>GPLGSPEFSKVPKEYRTAVSKAKQYASTVHMSKEELRSQLVSFDKYSQDASDYAVENSGIDYNKQALEKAKQYQDTLSMSPDAIRDQLVSFDKFTQEEADYAVANLK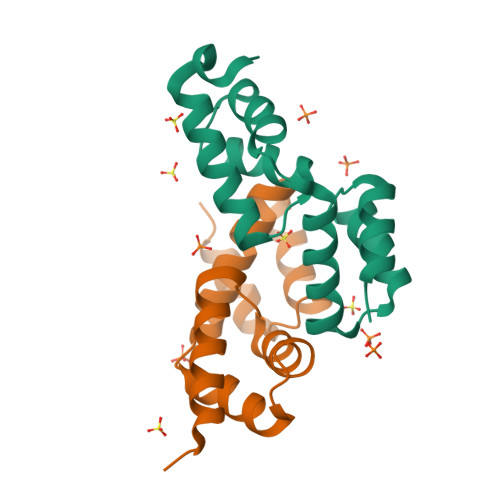[2x]>[4x]MQKLLSLPSNLVQSFHELERVNRTDWFCTSDPVGKKLGSGGGTSWLLEECYNEYSDGATFGEWLEKEKRILLHAGGQSRRLPGYAPSGKILTPVPVFRWERGQHLGQNLLSLQLPLYEKIMSLAPDKLHTLIASGDVYIRSEKPLQSIPEADVVCYGLWVDPSLATHHGVFASDRKHPEQLDFMLQKPSLAELESLSKTHLFLMDIGIWLLSDRAVEILMKRSHKESSEELKYYDLYSDFGLALGTHPRIEDEEVNTLSVAILPLPGGEFYHYGTSKELISSTLSVQNKVYDQRRIMHRKVKPNPAMFVQNAVVRIPLCAENADLWIENSHIGPKWKIASRHIITGVPENDWSLAVPAGVCVDVVPMGDKGFVARPYGLDDVFKGDLRDSKTTLTGIPFGEWMSKRGLSYTDLKGRTDDLQAVSVFPMVNSVEELGLVLRWMLSEPELEEGKNIWLRSEHFSADEISAGANLKRLYAQREEFRKGNWKALAVNHEKSVFYQLDLADAAEDFVRLGLDMPELLPEDALQMSRIHNRMLRARILKLDGKDYRPEEQAAFDLLRDGLLDGISNRKSTPKLDVYSDQIVWGRSPVRIDMAGGWTDTPPYSLYSGGNVVNLAIELNGQPPLQVYVKPCKDFHIVLRSIDMGAMEIVSTFDELQDYKKIGSPFSIPKAALSLAGFAPAFSAVSYASLEEQLKDFGAGIEVTLLAAIPAGSGLGTSSILASTVLGAINDFCGLAWDKNEICQRTLVLEQLLTTGGGWQDQYGGVLQGVKLLQTEAGFAQSPLVRWLPDHLFTHPEYKDCHLLYYTGITRTAKGILAEIVSSMFLNSSLHLNLLSEMKAHALDMNEAIQRGSFVEFGRLVGKTWEQNKALDSGTNPPAVEAIIDLIKDYTLGYKLPGAGGGGYLYMVAKDPQAAVRIRKILTENAPNPRARFVEMTLSDKGFQVSRS

In bacteria and plants, the two independent catalytic reactions in the salvage pathway can be accomplished by a single enzyme, the fucokinase/GDP-fucose pyrophosphorylase (FKP). FKP can convert l-fucose into GDP-fucose via a fucose-1-phosphate (Fuc-1-P) intermediate, and has been applied to the chemical synthesis of fucose-containing glycans and glycoconjugates. Each monomer is composed of an N-terminal GDP-fucose pyrophosphorylase domain, a C-terminal fucokinase domain and a linker in between.

We overexpressed and purified the full-length wild type FKP from Bacteroides fragilis 9343. In the end, we got a cyro-EM structure of the full-length FKP at 4.0 Å resolution with a C1 symmetry. The final structure model contains 810 amino acids, from residue 71 to 398 and 467 to 949. The overall structure of FKP exhibits a tetrameric organization. The tetrameric organization of FKP is mediated mainly by the CTDs. Two interfaces are identified in the structure, with one interface formed by a six-stranded β sheet interaction and the other by a loop-helix interaction. The GDP-fucose pyrophosphorylase domain contains a typical Rossmann fold and a left-handed β-helix fold. The fucokinase domain of FKP, as predicted, adopts a GHMP sugar kinase fold. G76A, R80A, G88A and K89A mutants almost completely lose their GDP-fucose pyrophosphorylase activities. Taken together, it strongly suggests that this loop region is critical to the GDP-fucose pyrophosphorylase activity of FKP and may be the putative GTP binding site during catalysis. For the glycine-rich motifs, result shows that the T602A, G757A and G902A mutants have greatly reduced fucokinase activities, while mutants with R592A, D594A, G597A, G598A, D601A, G758A, G759A, Q761A, D762A, G899A and G901A, respectively, retain hardly any fucokinase activities. This suggests that this large pocket surrounded by the highly conserved residues is a potential substrate-binding site in the fucokinase domain of FKP.>MPRKKDQVTKNDDGNQTSDVQTQDFKTAVQPDTNTAQLIKTYSNPKQRGDKGEIIYDGGLSSKLADVVDKTTEPHNADGAVKDGRIAPVKLDLEKQKLDKLKLFETSPFDPLTIKNNQDVVDKLYATQSSSIQEVVPTKTFATELQFGVTSEDMAKIYGAVAAVSKNVNSSVTYEVKRGTHELIKVPTIPHNLVLIQSDNGKHALIKEDLGQWPVETGISLVNQAGVFAVQLANKLGIDKPFVLDAGSNYFTDTSFIDTRKYCTDGLSPREIQKALNRQRAYYDRPELTISENKTLLSQSIIYPDADGNDVSIIFSGAMSHAIFTYAQSQWNKNIIKLDDYIREITLTVPKQYRPRRFKEIEHTHGYVYRELNQGSLLPLVDANLKESSSYYFKKLMSSISNVPVDARTLQSATAALAADTGQAVNRAQHVSMLTNRLTTANAPTVRAITVLTCMFKQFRIGMTYALDPNIMDVAAATCMLLFRPAQSISDEQYRYCLQTMAVFLTNTTYDIVNNDTIDVLKMKLRNQGWPFVERYNAVEIDMSVEPLRSPGQVGRYYNPFNIDPLTKKHVEDRLEEFINQVQVGRFRNASGNAVGTTLAAFLRACRDKTSANWRGYSVLVSRYRSLIPNELFESLRNISGEYNINPQDEHSFFFALAQINADDEFIGAIDKESAEYLDEYATLARDISNSLTLVKAAFGPLERTSGSIINHANNLNKVINHVFADKPLISETMLKILTIDGTTGKDGYRNWLDKLVGHNYPVYVEPVVNIMNFISARFVADSSYFGYTNEIMIMPNHINVPVDDRFGFRDSPFCTSLPRTIMGNDVRRISYNVFSMMEDIDDVISEGFILYDAYFNFSYDIMTTDGVTRLKEDILIVTDTGNDIKPIHFYIYFENRNDKKLRYESKMNVSYRLYIKTPACLLPLSDYMRAQHDYVSPSSSRVYIKDPAVVYTRS[2x];>MANRATSAFLDNPHPVGVNYVDEGSRQFVAVAELLASKLIDSSRESDESNSDVPFVQAYSKFADDNPRHLRVKTGGKMANALTNVIRSYYSINAPAIVPQVEIDRLASKATVSGDMYNSYAIFNSVPIVEVLSPARTTVSIVGSDRADVTMLNTGAGAANITFNFGQIAETVILKGSVPFQLARLNQPMPAARFTYKLRPLDGPFIVVLPVGNPLVISATAATRIQVPLAFNKALVESGFQTAMNDGLFDIQNVNYYSSFDEFIISQYHAQDGINRVSTCVILGLALQAYDQMRRALPVRR[13x];>MDVLSKGSLKELLAHLEKTPLEEAISYRIGTVPYQNVLISRNEYYNQLYPDTTSLIDGVSREGQRNVNGLIMSIISYVVSGSGHYIPNIGFMLLRRSILDILTKHDTGLVTNNLNYGIIARNLTVSKMNCEQRKRMLICFKLLAYKDGNQNDYEIYLNQNIPLKQIAPNFIPGDMRTVIHNQDQLAIVGIPAYRLTQSTELSIRDDNAKSYKLGYVDWYNSNSFLRERSEFNLIRLKDRDTKYGKLNGW[2x];>[6x]MAWVTQAYSSGLSQNSIISLTGNDRTVADGTFNSMIMPRAVIANEREHFMKTRIDKIEHDLNRSAKQEMMDRQSLAEDYNALNLAVGQEIKLDIATQHQLNRLGSAMYKADHERETELTDLINRIRENEVTVNGILENQKAITAAERADLLLEVVASTAKSVSAAGRAAADGSGVVPVFGPSVANGIKVGIDIADSVAEAAIAVKESGIITQLNDVYHAFQSVHVAPNDVIKPAAVVAGTSTELIGNLQAIYSRLRSHSDIGFKKATVGDVIPNSYMIKPVNSTEYASWQLYVIHPVQGSLGLVVQLMGDALTYNVFAQYGNTSASEFGKTVLTGGATNTALEGTKVKFQTKVTAQQALALTMALKDAASMLSQGELIGYFEQYINLALEPDNLSLQDNMHKYHHLLTSQNSPIDWNYHDEEMHKWLDSRKTTNYDAMQKKDGTVIADIHIPKVFNDLRNTTLHCKLEGKQTIAGYTVYEYLIGPWAHYGDIDYSVVVDTLNEETKWYCEVIGIDGHLLIEKSVQHKPEKILELTVNDSGVTSFNGRNHDRLKLKVYVKDSLSVKVFRNWIGINAPRVKTKMFNDHIGVKYDYSHFDKNISPAHLTLTDLGWHTWDQYNAGNWTNIKP;>MLSETELRALKKLSTTTSRVVGDSTLALPSNVKLSKGEVEKIAVTKKEMFDELAQCNLPTIELITREHTFNGDVIRFAAWLFLMNGQKLMIANNVAVRMGMQYATNLAGNNVKITYVTSNNVVKLGHIAAGVLANPYSNKGSGLFITYEYNLISNLIETGKVCVLFITSLSTTASSTNSFAYSTCSVPIENWDFNMIKLTAETSCASLTAMTNLVNSLVPGERTRPVGLYVDIPGVTVTTSASSGSLPLTTIPAVTPLIFSAYTKQVEEVGVINTLYALSYLP[6x]

Banna virus (BAV) is the prototype Seadornavirus, a class of reoviruses for which there has been little structural study. Here, we report atomic cryo-EM structures of three states of BAV virions—surrounded by 120 spikes (full virions), 60 spikes (partial virions), or no spikes (cores). In the full and partial BAV virions, genomic dsRNA segments and a number of RNA-dependent RNA polymerases (RdRps, VP1) are packaged in a double-layered icosahedral capsid consisting of three proteins (VP2, VP8, and VP10). The spikes protruding from the outer capsid shell are heterohexamers composed of a VP4 trimer capped by a VP9 trimer.

Visual inspection and 2D class averaging of purified BAV YN15-126-01 virions on cryo-EM micrographs revealed two types of virions: one surrounded by more spikes on the viral surface (hereafter referred to as full particles), and the other with sparser spiky density (partial particles). The ratio of full to partial particles was approximately 3:1. Icosahedral reconstructions of full and partial BAV particles (at ~5.7 Å resolution) revealed that they share overall structural features except for the different number of spikes on the virus surface. In the full BAV virions, there are 60 spikes sitting on VP10A and VP10B, respectively, while in the partial virions, there are only 60 spikes on VP10A. The thicker outer capsid shell is composed of 780 copies of VP8 and 120 copies of VP10, with each VP10 molecule being surrounded by six VP8 trimers. Two VP10 molecules are identified in each ASU, VP10A (closer to the icosahedral fivefold axis) and VP10B (closer to the threefold axis). In contrast, in the double-layered full BAV particles, 120 spikes made up of a VP4 trimer (for membrane penetration) and VP9 (for receptor binding) emanate from VP10 located at both type II and type III channels. The binding affinity of spikes at the two channels appears different, resulting in detachment of half the spikes when the partial particles form. BAV entry into the cell is a highly ordered process with stepwise detachment of viral spikes, as reflected by the variation in spike arrangement on full particles (120 spikes containing VP4 and VP9), partial particles (60 spikes containing VP4 and VP9), acidified particles (60 spikes containing VP4), and core particles (no spikes).>[2x]EPCVEVVPNITYQCMELNFYKIPDNLPFSTKNLDLSFNPLRHLGSYSFFSFPELQVLDLSRCEIQTIEDGAYQSLSHLSTLILTGNPIQSLALGAFSGLSSLQKLVAVETNLASLENFPIGHLKTLKELNVAHNLIQSFKLPEYFSNLTNLEHLDLSSNKIQSIYCTDLRVLHQMPLLNLSLDLSLNPMNFIQPG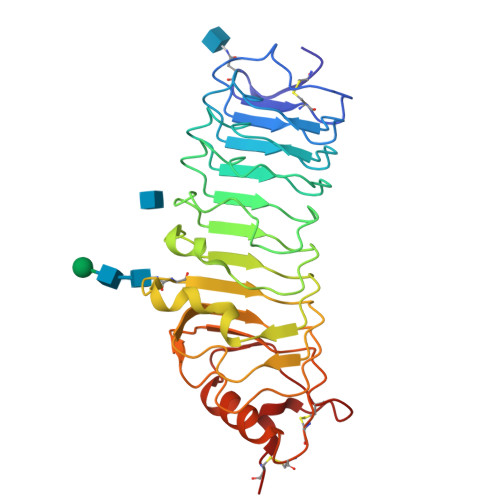AFKEIRLKELALDTNQLKSVPDGIFDRLTSLQKIWLHTNPWDCSCPRIDYLSRWLNKNSQKEQGSAKCSGSGKPVRSIICP;>[2x]QKQYWVCNSSDASISYTYCDKMQYPISINVNPCIELKGSKGLLHIFYIPRRDLKQLYFNLYITVNTMNLPKRKEVICRGSDDDYSFCRALKGETVNTTISFSFKGIKFSKGKYKCVVEAISGSPEEMLFCLEFVILHQPN> GLIVDTRDVEERVHVMRKTKLAPTVAHGVFNPEFGPAALSNKDPRLNEGVVLDEVIFSKHKGDTKMSAEDKALFRRCAADYASRLHSVLGTANAPLSIYEAIKGVDGLDAMEPDTAPGLPWALQGKRRGALIDFENGTVGPEVEAALKLMEKREYKFACQTFLKDEIRPMEKVRAGKTRIVDVLPVEHILYTRMMIGRFCAQMHSNNGPQIGSAVGCNPDVDWQRFGTHFAQYRNVWDVDYSAFDANHCSDAMNIMFEEVFRTEFGFHPNAEWILKTLVNTEHAYENKRITVEGGMPSGCSATSIINTILNNIYVLYALRRHYEGVELDTYT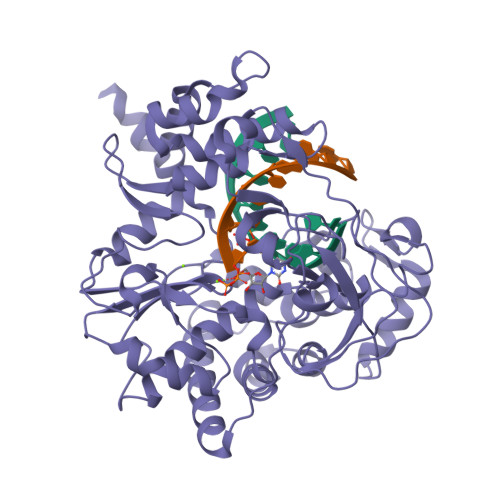MISYGDDIVVASDYDLDFEALKPHFKSLGQTITPADKSDKGFVLGHSITDVTFLKRHFHMDYGTGFYKPVMASKTLEAILSFARRGTIQEKLISVAGLAVHSGPDEYRRLFEPFQGLFEIPSYRSLYLRWVNAVCGDAAALEHH>MGMAPNMDAVADATAQVHVRNSHILEMHSDVLFHIGLTCSQEERQQVANTFGDVKFFITGGSAERMTHFAQSVAKELGITTPYGYQLAPIGSTSRYTLFKVGPVLVANHGIGMPSISILLHEVTKLLEYAGAHGATYIRMGTSGGIGVEPGTVVITSEGVNNKLESVDEVAVLGSTVRRPSICSPEVREEIITAAKEVGLPYAVGKTLSCNDFYEGQGRLDGAICEYTLEDKMAFLQKLADAGVRNIEMEARLMAGFCHKLNIPVAVVCVTLLNRLNGDQVLSSHETLQ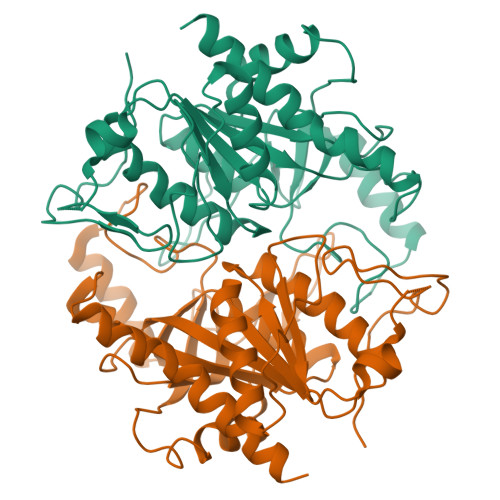DFERRPGAVLLHYIKSKVNASAAAALEHHHHHH[2x]>MAELLLVETPIPQQKHYESKPFPAVISPPSASIPIPALSLPLFTQTIKTQKHYLDSLLHESGAVLFRGFPVNSADDFNDVVEAFGFDELPYVGGAAPRTSVVGRVFTANESPPDQKIPFHHEMAQVREFPSKLFFYCEIEPKCGGETPIVLSHVVYERMKDKHPEFVQRLEEHGLLYVRVLGEDDDPSSPIGRGWKSTFLTHDKNLAEQRAVDLGMKLEWTEDGGAKTVMGPIPAIKYDESRNRKVWFNSMVAAYTGWEDKRNDPRKAVTFGDGKPLPADIVHDCLRILEEECVAVPWQRGDVLLIDNWAVLHSRRPFDPPRRVLA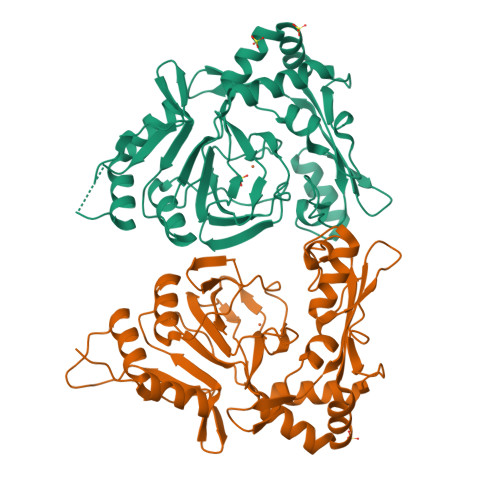SLCK[2x]> QSREIADNTY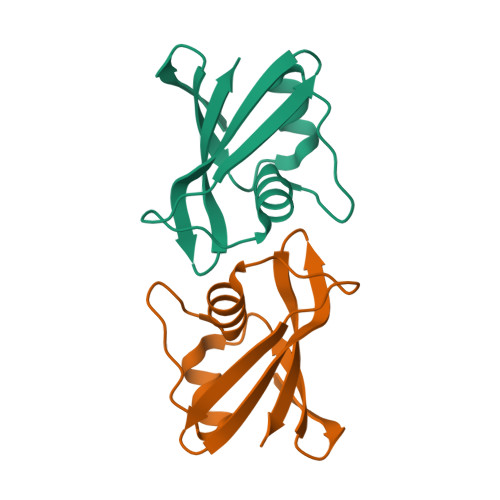IVLGTMTLNDFNEYFETDLESDNVDTIAGFYLTGVGTIPSQEEKEHFEVESNGKHLELINDKVKDGRVTKLKILVSE>SQDIVDFSQHPWKAPGPNDLRSPCPGLNTLANHGFLPRNGRNITIPMIVQAGFDGYNVQPDILILAAKVGLLTSPEPDTFTLDDLKLHGTIEHDASLSREDFALGDNLHFNEAIFNTLANSNPGSDVYNITSAGQVLKDRLADSLARNPNVTNTGKEFTIRTLE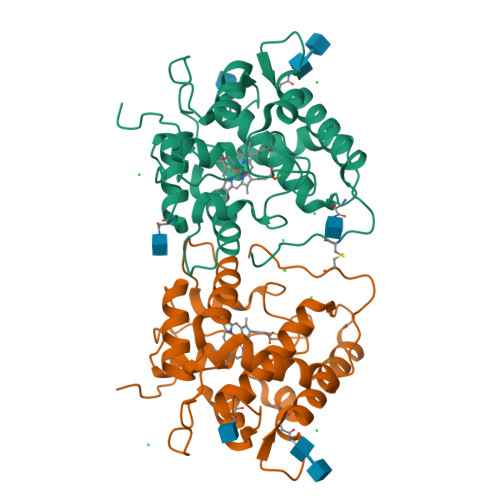SAFYLSVMGNATTGEAPKNFVQIFFREERLPIEEGWKRSTTPITSDTLNPIAGQISEASNWKPNPDQCPWIVLSPNL[2x]> GANNDMPVEQ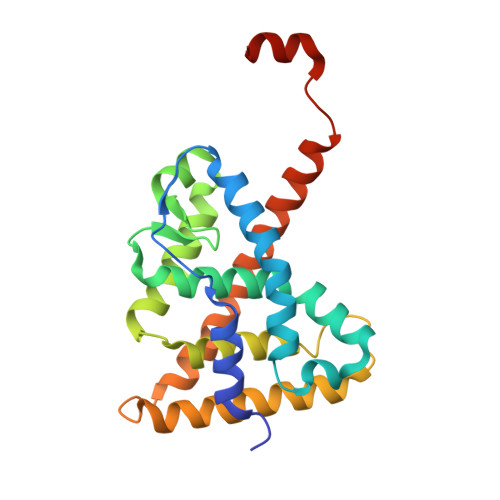ILEAELAVDPKIDTYIDAQKDPVTNICQAADKQLFTLVEWAKRIPHFTELPLEDQVILLRAGWNELLIAGFSHRSIMAKDGILLATGLHVHRSSAHQAGVGTIFDRVLTELVAKMRDMKMDKTELGCLRAVVLFNPDAKGLTAVQEVEQLREKVYASLEEYTKSRYPEEPGRFAKLLLRLPALRSIGLKCLEHLFFFKLIGDQPIDTFLMEMLENPSPAT>[4x]MHHHHHHLPNITILATGGDIAGGGDSATKSNYTVGKVGVENLVNAVPQLKDIANVKGEQVVNIGSQDMNDNVWLTLAKKINTDCDKTDGFVITHGVDTMEETAYFL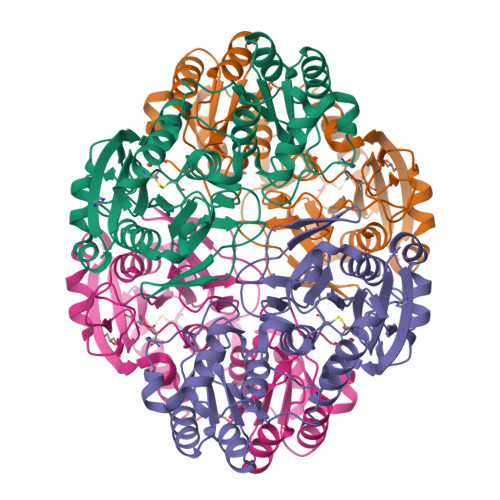DLTVKCDKPVVMVGAMRPSTSMSADGPFNLYNAVVTAADKASANRGVLVVMNDTVLDGRDVTTTNTTDVATFKSVNYGPLGYIHNGKIDYQRTPARKHTSDTPFDVSKLNELPKVGIVYNYANASDLPAKALVDAGYDGIVSAGVGNGNLYKSVFDTLATAAKTGTAVVRSSRVPTGATTQDAEVDDAKYGFVASGTLNPQKARVLLQLALTQTKDPQQIQQIFNQY> KET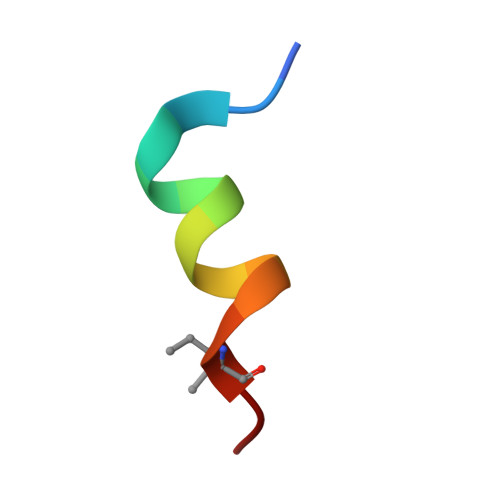AAAKFERQHVDS> MGHHHHHHHHHHSSGHIDDDDKHMEKSRPNLPQAVVGTGWTSKGQITVLDMHPGSGKTHRVLPELIRQCIDRRLRTLVLAPTRVVLKEMERALNGKRVRFHSPAVSDQQAGGAIVDVMCHATYVNRRLLPQGRQNWEVAIMDEAHWTDPHSIAARGHLYTLAKENKCALVLMTATPPGKSEPFPESNGAITSEERQIPDGEWRD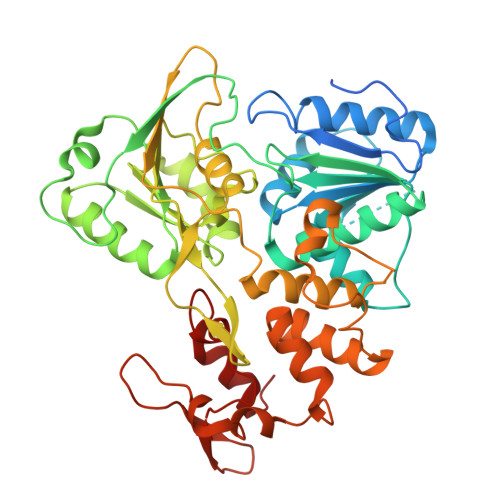GFDWITEYEGRTAWFVPSIAKGGAIARTLRQKGKSVICLNSKTFEKDYSRVRDEKPDFVVTTDISEMGANLDVSRVIDGRTNIKPEEVDGKVELTGTRRVTTASAAQRRGRVGRQDGRTDEYIYSGQCDDDDSGLVQWKEAQILLDNITTLRGPVATFYGPEQDKMPEVAGHFRLTEEKRKHFRHLLTHCDFTPWLAWHVAANVSSVTDRSWTWEGPEANAVDEASGDLVTFRSPNGAERTLRPVWKDARMFKEGRDIKEFVAYASGRR[4-[[[(2~{S})-2-[[2,3-bis(oxidanyl)phenyl]carbonylamino]-3-[[(2~{S})-2-[[2,3-bis(oxidanyl)phenyl]carbonylamino]-3-[2-[[2,3-bis(oxidanyl)phenyl]carbonylamino]ethanoylamino]propanoyl]amino]propanoyl]amino]methyl]-1,2,3-triazol-1-yl]methyl 4-[4-[(5~{S})-5-(acetamidomethyl)-2-oxidanylidene-1,3-oxazolidin-3-yl]-2-fluoranyl-phenyl]piperazine-1-carboxylate 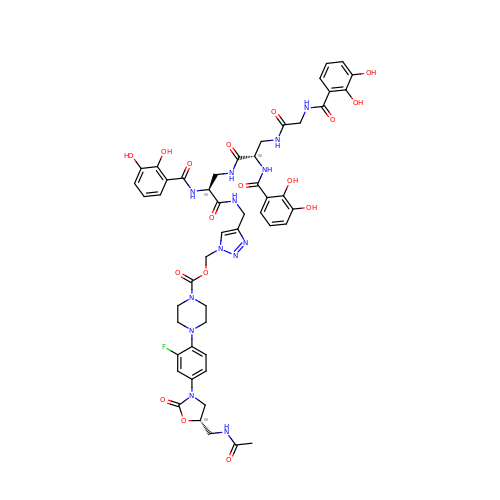| C50 H54 F N13 O17 | BNEIHKWYSZOFPI-LCFCVFAESA-N UDP-glucose 6-dehydrogenase (UGDH; EC 1.1.1.22) is the sole human enzyme that converts UDP-α-D-glucose (UDP-glucose) to UDP-α-D-glucuronic acid (UDP-glucuronic acid), an intermediate sugar in carbohydrate metabolism. Molecular cloning of hUGDH revealed it to be a 494-amino acid protein that shares 98% identity to bovine UGDH. hUGDH is a hexamer of 57-kDa subunits that assembles into a trimer of dimers. UGDH is a member of a small group of NAD+-dependent four-electron-transfer dehydrogenases. UGDH catalyzes two NAD+-dependent oxidations of UDP-glucose, the first reversible, to yield UDP-glucuronic acid in an overall irreversible process.

The structure of hUGDH in complex with NAD+ fragments and UDP-glucose was solved by molecular replacement and refined against 2.8 Å resolution data. The crystal asymmetric unit contains two open hexamers arranged as a closed dodecamer. Here, we have solved an alternate substrate-bound structure of hUGDH, which reveals the asymmetrical open hexameric quaternary conformation that was previously observed in the inhibitor-bound structure. The NAD+ molecules in the present open hexamer structure are partially disordered. In comparison to the closed hexamer, the open hexamer residues Ser130 and Thr131 have made a large switch toward the interior of the NAD+-binding site to occupy the space vacated by the disordered nicotinamide moiety and the absent catalytic water. In the open hexamer protomers there is no bound active water. Instead, Thr131 occupies the former location of the active water and causes Asp280 to turn away from the UDP-glucose. Arg260 situated in a loop within the central domain of one protomer reaches across to contact and position the glucose from the UDP-glucose within the second protomer. Hence, we propose that the present structure of hUGDH represents a trapped intermediate conformation that provides valuable insight into the reaction mechanism.

>[12x]MFEIKKICCIGAGYVGGPTCSVIAHMCPEIRVTVVDVNESRINAWNSPTLPIYEPGLKEVVESCRGKNLFFSTNIDDAIKEADLVFISVNTPTKTYGMGKGRAADLKYIEACARRIVQNSNGYKIVTEKSTVPVRAAESIRRIFDANTKPNLNLQVLSNPEFLAEGTAIKDLKNPDRVLIGGDETPEGQRAVQALCAVYEHWVPREKILTTNTWSSELSKLAANAFLAQRISSINSISALCEATGADVEEVATAIGMDQRIGNKFLKASVGFGGSCFQKDVLNLVYLCEALNLPEVARYWQQVIDMNDYQRRRFASRIIDSLFNTVTDKKIAILGFAFKKDTGDTRESSSIYISKYLMDEGAHLHIYDPKVPREQIVVDLSHPGVSEDDQVSRLVTISKDPYEACDGAHAVVICTEWDMFKELDYERIHKKMLKPAFIFDGRRVLDGLHNELQTIGFQIETIGKKVSSKRIPYAPSGEIPKFSLQDP>[6x]METSENKSEIKILSLNGGGVRGLFTITLLAELESIIEKREKCENVKIGDYFDLITGTAIGGILALGLASGKSARELKEAFEINATKIFPLKRFKNKQWWNLLRRSIYESEPLYDAVKSMIGETIKFEDLNRRVMITSVNLSTGKPKFFKTPHNPMFTMDREIRLIDAAMATSAAPTYFK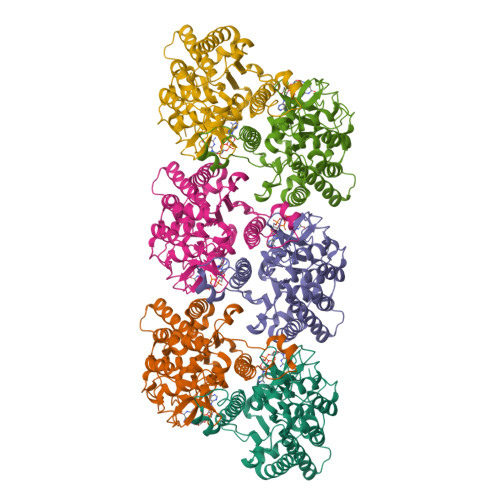PHYIEKLENYFADGGLVANNPSYIGIREVLIDMKNDFPDAKPENIKVLNIGTLSEDYCISPETLSKNSGKGYLSLWNMGERIVLSTMTANQHLQRFMLLREFEALKIEKNYVEIDETIPNEAAAEITLDNASEGCLKALRGSGKKLAAERYTKNEELRNFFLKKAEPFVPYIESSEVTAHHHHHH> HGHHSHGKPLTEVEQKAANGVFDDANVQNRKLSDWDGVWQSVYPLLQSGKLDPVFQKKADADKTKTFAEIKDYYH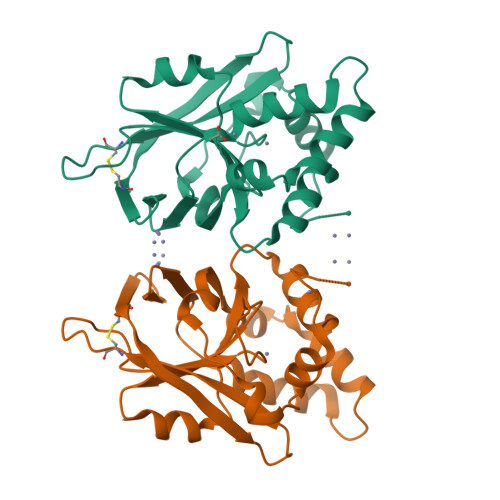KGYATDIEMIGIEDGIVEFHRNNETTSCKYDYDGYKILTYKSGKKGVRYLFECKDPESKAPKYIQFSDHIIAPRKSSHFHIFMGNDSQQSLLNEMENWPTYYPYQLSSEEVVEEMMSH>SYTLPSLPYAYDALEPHFDKQTMEIHHTKAHQTYVNNANAALESLPEFANLPVEELITKLDQLPADKKTVLRNNAGGHANHSLFWKGLKKGTTLQGDLKAAIERDFGSVDNFKAEFEKAAASRFGSGWAWLVLKGDKLAVVSTANQDSPLMGEAISGASGFPIMGLDVWE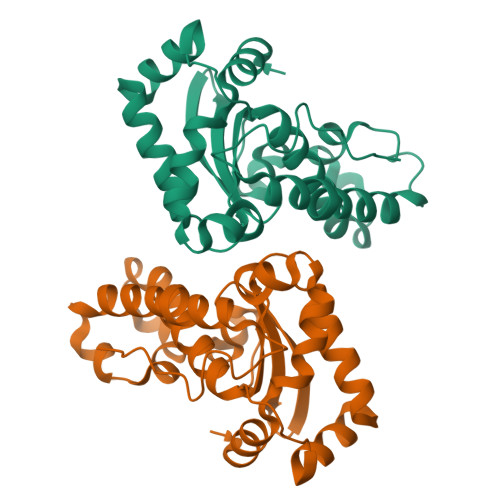HAYYLKFQNRRPDYIKEFWNVVNWDEAAARFAAKK[4x]>[4x]KESAAAKFERQHMDSGNSASSSSNYCNQMMCCRKMTQGKCKPVN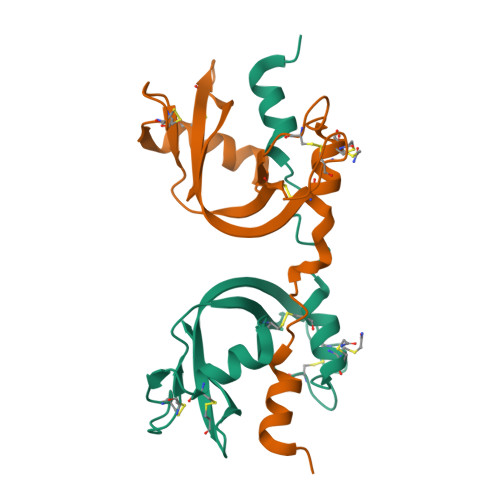TFVHESLADVKAVCSQKKVTCKDGQTNCYQSKSTMRITDCRETGSSKYPNCAYKTTQVEKHIIVACGGKPSVPVHFDASV>MGSDKIHHHH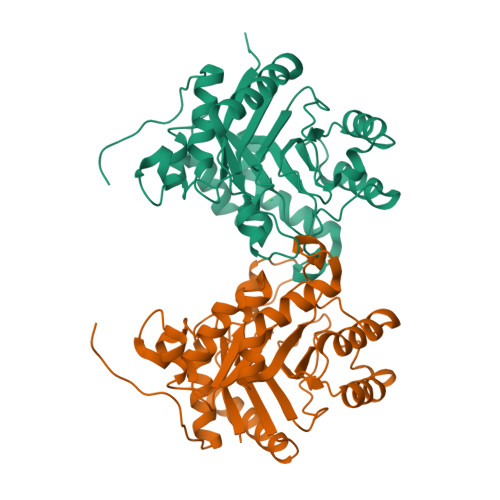HHMIRLGLTSFSEHDYLTGKKRSTLYEYASHLPLVEMDTAYYGIPPKERVAEWVKAVPENFRFVMKVYSGISCQGEWQTYYASEEEMITAFLESMAPLIESKKLFAFLVQFSGTFGCTKENVAYLQKIRHWFKDLPIAIELRNNSWYQPNFVKQMLQFMKENQFSLVIVDEPQIPTNPVPFYPYVTNPNLVLFRFHGRNAAGWLANDAEWRKKRTLYHYNTQEIADLSEAVLKMSQEAKEVGVIFNNNSGGDAAENALQMQKVLNLSYDDLNPKQLDLF[2x]>[2x]MEPLQDPAQIVARLEALASPVRLEIFRLLVEQEPTGLVSGDIAEHLGQPHNGISFHLKNLQHAGLVTVQREGRYQRYRAAMPVVRALVAYLTENCCHG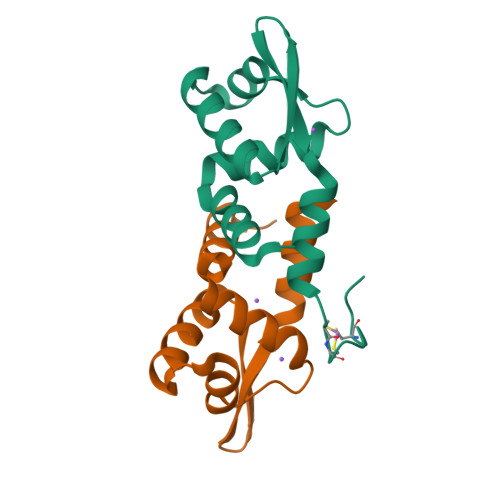TRDCALSGETRSPSVQEGNQHHHHHH> GV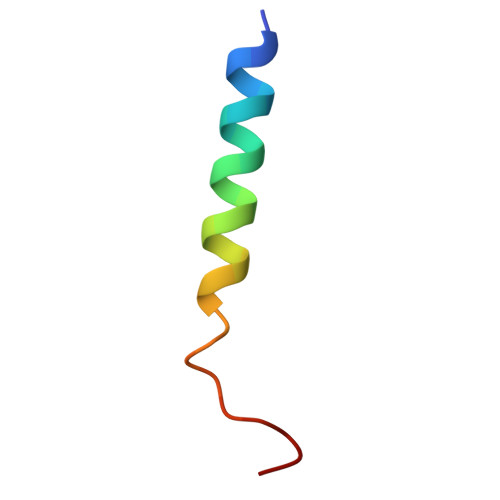TSEGKFDKFLEERAKAADRLPNLSS>SVVIVGKISFCPKDVLGHGAEGTIVYRGMFDNRDVAVKRILPECFSFADREVQLLRESDEHPNVIRYFCTEKDRQFQYIAIELCAATLQEYVEQKDFAHLGLEPITLLQQTTSGLAHLHSLNIVHRDLKPHNILISMPNAHGKIKAMISDFGLCKKLAVGRHSFSRRSGVPGTEGWIAPEMLSEDCKENPTYTVDIFSAGCVFYYVISEGSHPFGKSLQRQANILLGACSLDCLHPEKHEDVIARELIEKMIAMDPQKRPSAKHVLKHPFFWSLEKQLQFFQDVSDRIEKESLDGPIVKQLERGGRAVVKMDWRENITVPLQTDLRKFRTYKGGSVRDLLRAMRNKKHHYRELPAEVRETLGSLPDDFVCYFTSRFPHLLAHTYRAMELCSHERLFQPYYFHEPPEPQPPVTPDAL[2x]

IRE1 resides in the ER membrane. It has an N-terminal stress sensing domain in the ER lumen and a cytoplasmic kinase/ribonuclease domain which are connected by a single-pass transmembrane helix. The lumenal domains dimerise in response to ER stress bringing the cytoplasmic domains together. IRE1 then undergoes autophosphorylation, generating a specific endoribonuclease activity that hydrolyses 2 stem-loops in the pre-mRNA for a bZIP transcription factor.

Purified, dephosphorylated hIRE1 crystallized in the absence of nucleotide and diffraction data were collected to 2.6 Å. Our crystal structure shows apo-hIRE1 is a symmetrical dimer in a back-to-back conformation similar to the structure of phosphorylated yIRE1, and distinct from the face-to-face dimer previously observed in ADP-bound hIRE. While the unphosphorylated activation loop is not observed in our structure, the kinase active site has features associated with a functional kinase: the conserved Lys-Glu salt bridge between Lys599 in β3 and Glu612 in αC is formed; the side chains of Tyr628, Leu616, Phe712 and His686 form a continuous hydrophobic R-spine, although the side chain of Phe712 is mis-aligned; and the gatekeeper Ile642 packs against the αC-helix. However, in the apo-hIRE1 structure there is a large void between the RNase domains and only 227 Å2 is buried. However, in the apo-IRE1 structure there is a rotation of approximately 13° between protomers pivoting about a fulcrum at the interface in the N-lobe. The rotation keeps the N-lobes in close contact but leads to a ~ 10 Å displacement of residues within the RNase domain core. The contacts between monomers at the apo-hIRE1 dimer interface are symmetrical and mainly within the N-lobe. An extensive network of salt bridges and hydrogen bonds is formed between an acidic region at the C-terminal end of αC and β4 on one protomer and a basic protrusion formed by the β(−1)-β0 and β2-β3 loops on the opposing monomer. The activation loop is well defined from 711-726 and 732 onwards in the ligand-bound structure, whereas residues 713-731 are unresolved in the apo structure. The twist in apo-hIRE1 disengages the RNase domains, which might reflect lower RNase activity.>MDSDTLSGLLENVAKKFPDRRALSVSGKFNLTHARLHDLIERAASRLVSDAGIKPGDVVALTFPNTVEFVIMFLAVIRARATAAPLNAAYTAEEFEFYLSDSDSKLLLTSKEGNAPAQEAASKLKISHVTATLLDAGSDLVLSVADSDSVVDSATELVNHPDDGALFLHTSGTTSRPKGVPLTQLNLASSVKNIKAVYKLTESDSTVIVLPLFHVHGLLAGLLSSLGAGAAVTLPAAGRFSATTFWP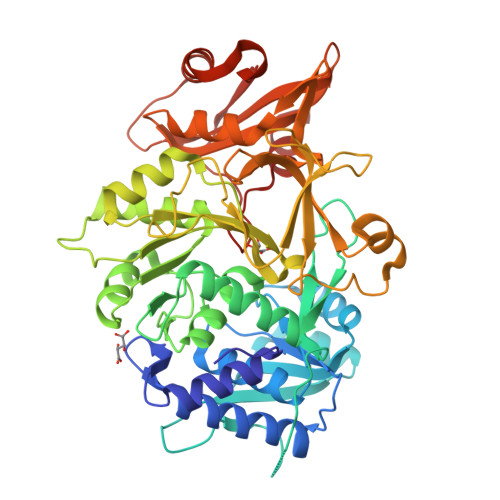DMKKYNATWYTAVPTIHQIILDRHASHPETEYPKLRFIRSCSASLAPVILSRLEEAFGAPVLEAYAMTEATHLMSSNPLPEEGPHKPGSVGKPVGQEMAILNEKGEIQEPNNKGEVCIRGPNVTKGYKNNPEANKAGFEFGWFHTGDIGYFDTDGYLHLVGRIKELINRGGEKISPIEVDAVLLTHPDVSQGVAFGVPDEKYGEEINCAVIPREGTTVTEEDIKAFCKKNLAAFKVPKRVFITDNLPKTASGKIQRRIVAQHFLEKP[2x]> MAMRLNEDLDDSGELHEINVTPFIDVMLVLLIIFMVAAPLATVDIRVDLPASSAKPQPRPEKPVFLSVK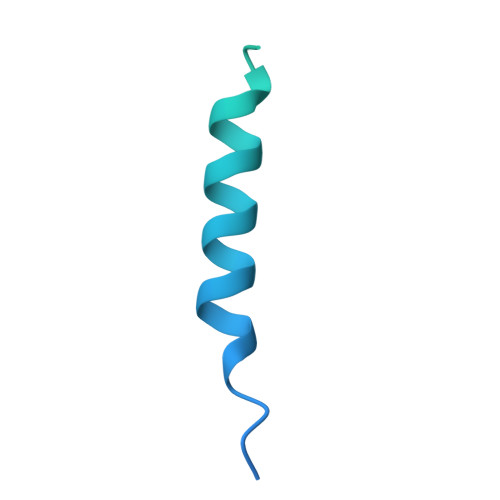ADKQLYVGDQPVNADQLTSVLDQRTQANKETTIFFQADKSVDYETLMSVMDTLRKAGYLKVGLVGMEGAAKHHHHHH methyl 6-deoxy-2-Se-methyl-2-seleno-alpha-L-galactopyranoside 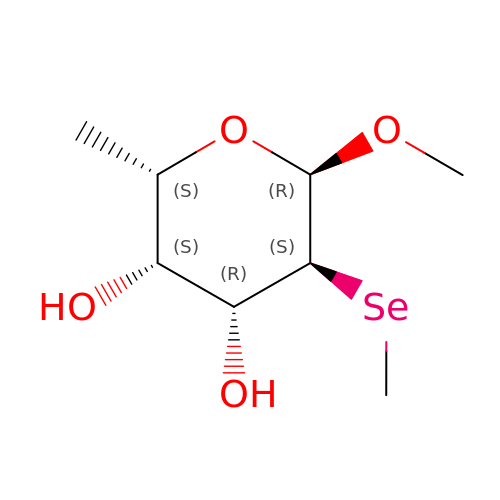| C8 H16 O4 Se | GFGVRXDXSFUDNW-FMGWEMOISA-N> MVARPKSEDKKQALLEAATQAIAQSGIAASTAVIARNAGVAEGTLFRYFATKDELINTLYLHLKQDLCQSMIMELDRSITDAKMMTRFIWNSYISWGLNHPARHRAIRQLAVSEKLTKETEQRADDMFPELRDLCHRSVLMVFMSDEYRAFGDGLFLALAETTMDFAARDPARAGEYIALGFEAMWRALTREEQ

The local transcriptional repressor RamR, which is located directly upstream of ramA, belongs to the TetR family of regulatory proteins and represses the expression of both ramA and ramR. Here, we report the crystal structure of RamR in complex with cholic and chenodeoxycholic acids. Both cholic and chenodeoxycholic acids decreased the DNA-binding affinity of RamR, resulting in increased transcription of ramA.

To elucidate the recognition mechanism of cholic and chenodeoxycholic acids by RamR, we determined the individual crystal structures of RamR complexed to both of these compounds. Electron density maps of each co-crystal structure are shown in Fig. 2b and these structures were refined to resolutions of 2.0 and 1.8 Å for cholic and chenodeoxycholic acids, respectively. RamR binds two molecules of either cholic or chenodeoxycholic acid per dimer. The structural difference between cholic and chenodeoxycholic acid lies in the presence or absence of a 12-hydroxyl group, which in turn results in a difference in the electron density maps of RamR bound to these compounds (indicated by red arrows). Comparison of the ligated structures with unligated RamR revealed that the binding of cholic or chenodeoxycholic acid triggers uncoiling of the α7b and α8a helices, suggesting that RamR recognizes these compounds via an induced-fit mechanism. Instead of a π–π interaction, both bile acids form four hydrogen bonds with the Tyr59, Thr85, Ser137 and Asp152 residues of RamR. The KD values obtained from SPR data for chenodeoxycholic and cholic acids were 65.3 µM and 60.5 µM, respectively. RamR protein solution was passed over the DNA fragment immobilized on a sensor chip while in the presence or absence of cholic or chenodeoxycholic acid (up to 500 µM). Both bile acids inhibited the binding of RamR to the DNA, in a concentration-dependent manner. The IC50 values of cholic and chenodeoxycholic acids derived from the SPR data were 33.0 µM and 19.2 µM, respectively.> LYFQGAMCYIIAKRFKKSGCVALKAKRGKELADFATDLQKKLGYDIQIVAITRPTAYGEYEPYKFVNSFE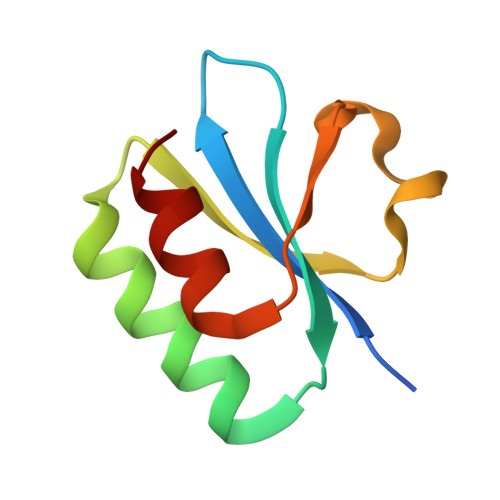EFSIEASRL3-[(2,4-dichlorophenyl)carbonylamino]-4-methoxy-~{N}-oxidanyl-benzamide 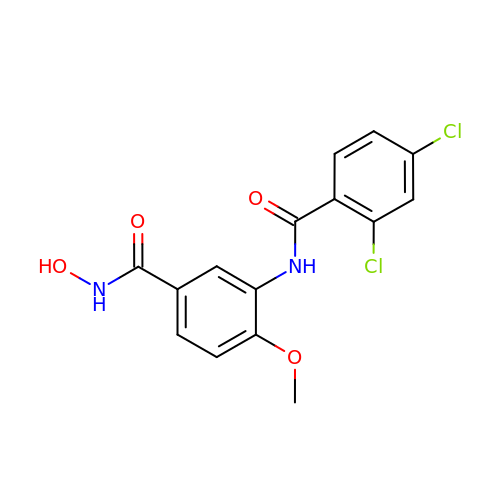| C15 H12 Cl2 N2 O4 | DSWXYOCCSDFQSQ-UHFFFAOYSA-N[(3S)-3-(4-bromo-1H-pyrazol-1-yl)pyrrolidin-1-yl][3-(propan-2-yl)-1H-pyrazol-5-yl]methanone 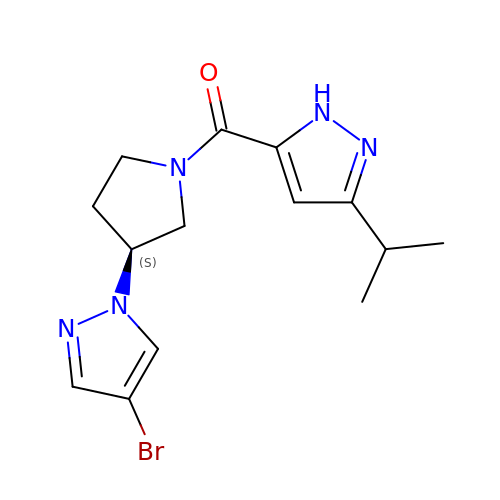| C14 H18 Br N5 O | JFPBFPWCRUXYRC-NSHDSACASA-N>[8x]MAHHHHHHMVATHTLADKVVLIAGGAKNLGGLIARDLAGHGAKAVAIHYNSAASQAQAEETAAAVRAAGAE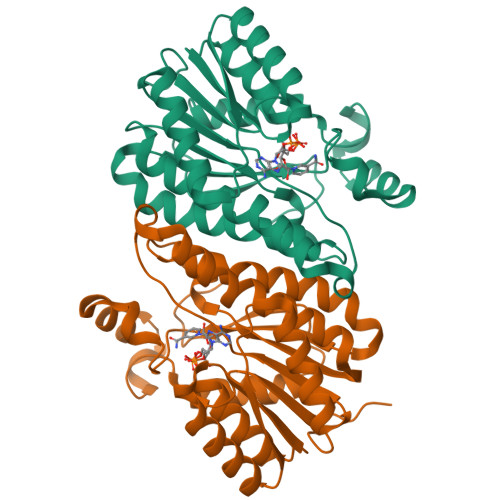AATFQADLTTAAAVEKLFDDAKQRFGKIDIAINTVGKVLKKPFTEISEAEYDEMFAVNSKSAFFFIKEAGRHLEDHGKLVTLVTSLLGAFTPFYAAYEGSKAPVEHFTRAASKEYGARGISVTAVGPGPMDTPFFYPAEGADAVAYHKTAAALSPFSKTGLTDIEDVVPFIRHLVTDGWWITGQTILINGGYTTK> DDQQLDHNFKQMEEHLALM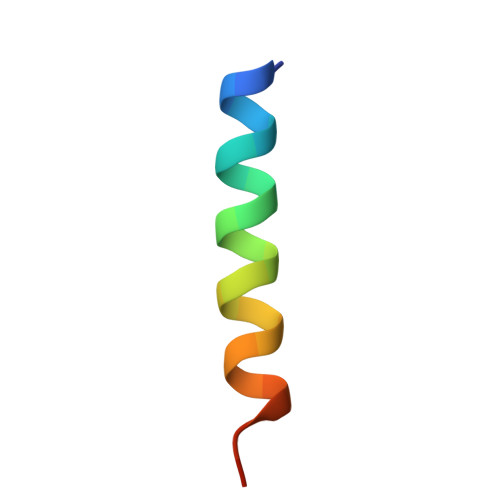VEGNE>[2x]MRVITLAGSPRFPSRSSSLLEYAREKLNGLDVEVYHWNLQNFAPEDLLYARFDSPALKTFTEQLQQADGLIVATPVYKAAYSGALKTLLDLLPERALQGKVVLPLA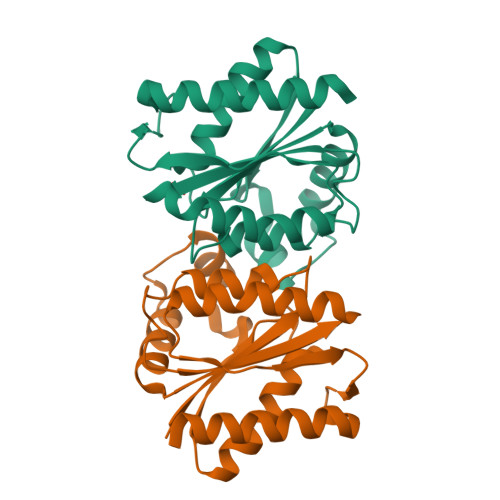TGGTVAHLLAVDAALKPVLSALKAQEILHGVFADDSQVIDYHHRPQFTPNLQTRLDTALETFWQALHRRDVQVPDLLSLRGNAHA>MMRYRKGARDTAFLVLYRWDLRGENPGELFKEVVEEKNIKNKDAYEYAKKLVDTAVRHIEEIDSIIEKHLKGWSIDRLGYVERNALRLGVAELIFLKSKEPGRVFIDIVDLVKKYADEKAGKFVNGVLSAIYKAYITSSKEEKPSLKSE[2x];>[2x]GMEQEKIRIKLRAYDHRLLDQSVKQIIETVKRTGGVVKGPIPLPTRKSEFSRILDIIRFTPQT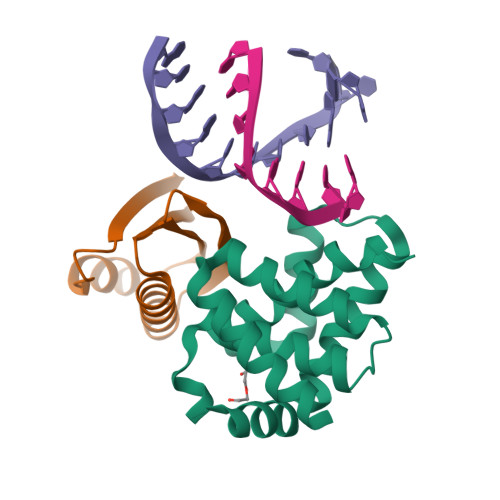IEALMEISLPAGVDVEVKMRG The flagellum is the most prominent extracellular structure in bacteria, with a molecular weight in the hundreds of megadaltons. Structurally, the flagellum can be divided into three major components: basal body, hook and filament. A ring-like structure formed by the proteins FlgK and FlgL, termed the hook–filament junction (HFJ), forms the connection between the flexible hook and the rigid filament. To assemble a filament, flagellin monomers are secreted through the flagellar basal body and hook, and polymerize at the distal end.

Using our short-flagellum cryo-EM dataset, we were able to determine the structure of the intact HFJ, anchored to both the hook and the filament, to 2.9 Å resolution. In this structure, both FlgK and FlgL form 11-mer layers that separate the hook protein FlgE from the filament protein FliC. These components—FlgE, FlgK, FlgL and FliC—are aligned to form a continuous protofilament along the 11-start symmetry axis. A total of 11 FlgL subunits form the distal HFJ layer beneath the filament, while 11 FlgK subunits form the proximal layer above the hook. As previously observed for the hook, the protofilaments in the junction can be structurally classified into two types: extended and compressed. Substantial structural shifts occur in FlgK, FlgL and FlgE subunits when transitioning from the extended to the compressed state, while the shift in flagellin subunit FliC remains minimal. Notably, FliC shows no substantial shift, suggesting that the HFJ prevents mechanical force transmissions to the filament. We propose that the HFJ functions as a mechanical buffer, leveraging the elasticity of FlgK to prevent mechanical stress from propagating to the flagellin filament. In conclusion, our results indicate that, while the interface appears relatively robust towards mutations, the integrity of the FlgKL interface is crucial for maintaining motility in S. enterica.

>MSFSQAVSGLNAAATNLDVIGNNIANSATYGFKSGTASFADMFAGSKVGLGVKVAGITQDFTDGTTTNTGRGLDVAISQNGFFRLVDSNGSVFYSRNGQFKLDENRNLVNMQGMQLTGYPATGTPPTIQQGANPAPITIPNTLMAAKSTTTASMQINLNSTDPVPSKTPFSVSDADSYNKKGTVTVYDSQGNAHDMNVYFVKTKDNEWAVYTHDSSDPAATAPTTASTTLKFNENGILESGGTVNITTGTINGATAATFSLSFLNSMQQNTGANNIVATNQNGYKPGDLVSYQINNDGTVVGNYSNEQEQVLGQIVLANFANNEGLASQGDNVWAATQASGVALLGTAGSGNFGKLTNGALEASNVDLSKELVNMIVAQRNYQSNAQTIKTQDQILNTLVNLR[13x];>[11x]MSSLINHAMSGLNAAQAALNTVSNNINNYNVAGYTRQTTILAQANSTLGAGGWIGNGVYVSGVQREYDAFITNQLRGAQNQSSGLTTRYEQMSKIDNLLADKSSSLSGSLQSFFTSLQTLVSNAEDPAARQALIGKAEGLVNQFKTTDQYLRDQDKQVNIAIGSSVAQINNYAKQIANLNDQISRMTGVGAGASPNDLLDQRDQLVSELNKIVGVEVSVQDGGTYNLTMANGYTLVQGSTARQLAAVPSSADPTRTTVAYVDEAAGNIEIPEKLLNTGSLGGLLTFRSQDLDQTRNTLGQLALAFADAFNAQHTKGYDADGNKGKDFFSIGSPVVYSNSNNADKTVSLTAKVVDSTKVQATDYKIVFDGTDWQVTRTADNTTFTATKDADGKLEIDGLKVTVGTGAQKNDSFLLKPVSNAIVDMNVKVTNEAEIAMASESKLDPDVDTGDSDNRNGQALLDLQNSNVVGGNKTFNDAYATLVSDVGNKTSTLKTSSTTQANVVKQLYKQQQSVSGVNLDEEYGNLQRYQQYYLANAQVLQTANALFDALLNIR;>[11x]MRISTQMMYEQNMSGITNSQAEWMKLGEQMSTGKRVTNPSDDPIAASQAVVLSQAQAQNSQYALARTFATQKVSLEESVLSQVTTAIQTAQEKIVYAGNGTLSDDDRASLATDLQGIRDQLMNLANSTDGNGRYIFAGYKTEAAPFDQATGGYHGGEKSVTQQVDSARTMVIGHTGAQIFNSITSNAVPEPDGSDSEKNLFVMLDTAIAALKTPVEGNNVEKEKAAAAIDKTNRGLKNSLNNVLTVRAELGTQLSELSTLDSLGSDRALGQKLQMSNLVDVDWNSVISSYVMQQAALQASYKTFTDMQGMSLFQLNR;>[15x]MAQVINTNSLSLLTQNNLNKSQSALGTAIERLSSGLRINSAKDDAAGQAIANRFTANIKGLTQASRNANDGISIAQTTEGALNEINNNLQRVRELAVQSANSTNSQSDLDSIQAEITQRLNEIDRVSGQTQFNGVKVLAQDNTLTIQVGANDGETIDIDLKQINSQTLGLDTLNVQQKYKVSDTAATVTGYADTTIALDNSTFKASATGLGGTDQKIDGDLKFDDTTGKYYAKVTVTGGTGKDGYYEVSVDKTNGEVTLAGGATSPLTGGLPATATEDVKNVQVANADLTEAKAALTAAGVTGTASVVKMSYTDNNGKTIDGGLAVKVGDDYYSATQNKDGSISINTTKYTADDGTSKTALNKLGGADGKTEVVSIGGKTYAASKAEGHNFKAQPDLAEAAATTTENPLQKIDAALAQVDTLRSDLGAVQNRFNSAITNLGNTVNNLTSARSRIEDSDYATEVSNMSRAQILQQAGTSVLAQANQVPQNVLSLLR>QRAGNETPENHPPLTWQRCTAPGNCQTVNAEVVIDANWRWLHDDNMQNCYDGNQWTNACSTATDCAEKCMIEGAGDYLGTYGASTSGDALTLKFVTKHEYGTNVGSRFYLMNGPDKYQMFNLMGNELAFDVDLSTVECGINSALYFVAMEEDGGMASYPSNQAGARYGTGYCDAQCARDLKFVGGKANIEGWKSSTSDPNAGVGPYGSCCAEIDVWESNAYAFAFTPHACTTNEYHVCETTNCGGTYSEDRFAGKCDANGCDYNPYRMGNPDFYGKGKTLDTSRKFTVVSRFEENKLSQYFIQDGRKIEIPPPTWEGMPNSSEITPELCSTMFDVFNDRNRFEEVGGFEQLNNALRVPMVLVMSIWDDHYANMLWLDSIYPPEKEGQPGAARGDCPTDSGVPAEVEAQFPDAQVVWSNIRFGPIGSTYDF[4x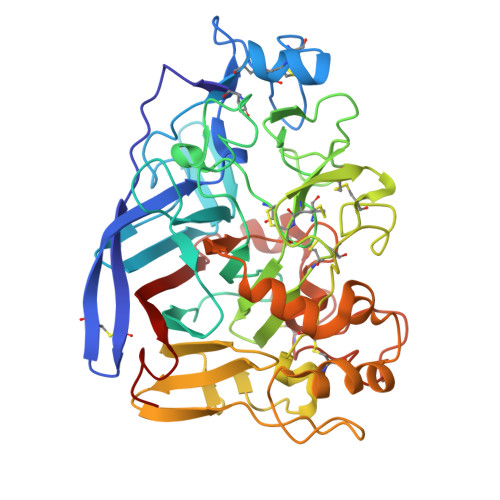]>MSKKDSKYKMSHTFESRQSDAAKVRERHPDRLPIICEKVYNSDIGELDRCKFLVPSDLTVGQFVSVLRKRV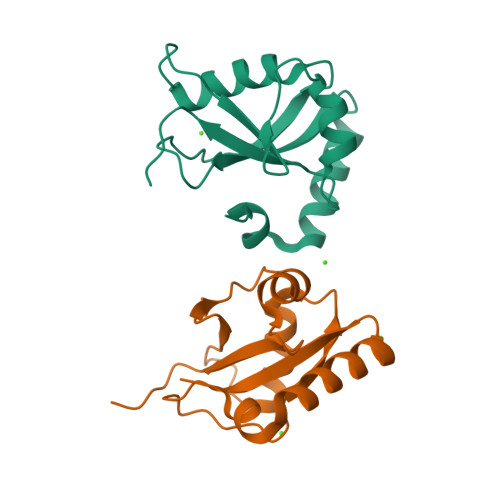QLEAESALFVYTNDTVLPSSAQMADIYSKYKDEDGFLYMKYSGEATFG[2x]> MQLSKEPRELNREWLIVLSELGQGAFGIVYEASLSEPKAPEIQVAAKSLRKDAMDNEREELLEEALVMAQMEHANVVGLIGVITKGRPIYVVLEHMRNGSLKDYVMNKTCTPAQQVTWSRQVASGMAHIHSLGFIHRDLAARNVLLSASLTAKVADFGLARESTDDAYYRSRGGNVPVRWTAPEALEDNIFSEKSDVWAFGVLMYEVYTKAAMPYTGWNNQRVWIEVTNGFRLPCPADCPLPVFKIMSMCWLHDRHERPSFETLVKALAALETDSDMSSLFQS

Receptor tyrosine kinases are crucial signaling molecules in animal cells, regulating inter-cellular responses to extracellar signals via numerous different pathways dependent on the organism involved. These receptors consist of an extracellular ligand-binding domain, a single transmembrane helix, and a cytoplasmic tyrosine kinase domain. The choanoflagellate M. brevicollis contains 128 protein kinases, including 88 receptor tyrosine kinases. The kinase described in this study is from the M. brevicollis receptor tyrosine kinase C (RTKC) family.

We determined the crystal structure at 1.95 Å resolution of the kinase domain of the M. brevicollis receptor tyrosine kinase C8 (RTKC8, a member of the choanoflagellate receptor tyrosine kinase C family) bound to the kinase inhibitor staurospaurine. The RTKC8 kinase domain is in an active conformation, with two staurosporine molecules bound to the kinase, one at the active site and another at the peptide-substrate binding site. The RTKC8 kinase crystallized in an active conformation with a RMSD of 1.0 Å over 201 Cα atoms to the structure of Lck in an active conformation. The conserved Glu 1592 of the αC-helix is rotated towards the active site to form a salt bridge with Lys 1575 of the β3-strand, oriented as “αC-helix-in”. The kinase is crystallized in “DFGin” conformation where the DFG-Asp is pointed towards the active site and the DFG-Phe interacts with the αC-helix. The tyrosine residues which would be expected to be phosphorylated in the activation loop (Tyr 1697 and Tyr 1698) were in the disordered activation loop region. There are three hydrogen bonds, with Glu 1622, Met 1624 and Arg 1670 and five hydrophobic interactions, with Leu 1549, Val 1557 and Ala 1573 from N-lobe, and Gly 1627 and Leu 1673 from C-lobe. Another molecule of staurosporine was found bound to the C-lobe of the kinase domain in a hydrophobic groove between the activation loop, the αEF helix and the αG helix. The ligand interacts with hydrophobic residues (Gly 1701, Gly 1702, Val 1704, Val 1706) in the activation loop and Trp 1752, Asn 1748 and Gln 1749 in the αG-helix. The purified RTKC8 kinase is catalytically active and can phosphorylate tyrosine residue containing peptides generated from its C-terminal tail sequence.> MGGAHKVRAGGPGLERAEAGVPAEFSIWTREAGAGGLAIAVEGPSKAEISFEDRKDGSCGVAYVVQEPGDYEVSVKFNEEHIPDSPF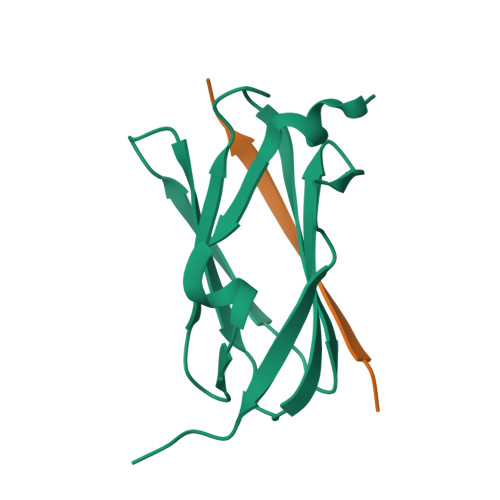VVPVASPSGGGGGG;> ARIKAINTFFAKN> RAKVAMSHFEPHEYIRYDLLEKNIDIVRKRLNRPLTLSEKIVYGHLDDPANQEIERGKTYLRLRPDRVAMQDATAQMAMLQFISSGLPKVAVPSTIHCDHLIEAQLGGEKDLRRAKDINQEVYNFLATAGAKYGVGFWRPGSGIIHQIILENYAYPGVLLIGTDSHTPNGGGLGGICIGVGGADAVDVMAGIPWELKCPKVIGVKLTGSLSGWTSPKDVILKVAGILTVKGGTGAIVEYHGPGVDSISCTGMATICNMGAEIGATTSVFPYNHRMKKYLSKTGRADIANLADEFKDHLVPDPGCHYDQVIEINLSELKPHINGPFTPDLAHPVAEVGSVAEKEGWPLDIRVGLIGSCTNSSYEDMGRSAAVAKQALAHGLKCKSQFTITPGSEQIR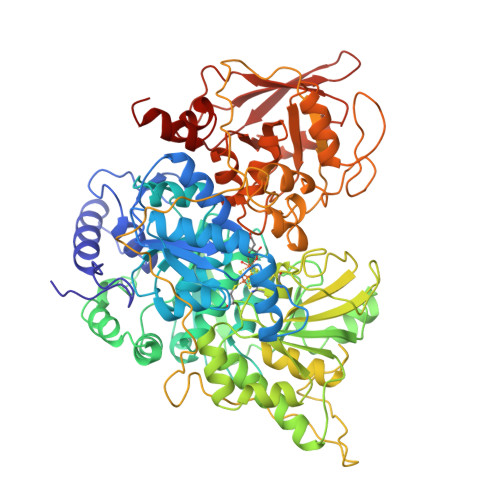ATIERDGYAQVLRDVGGIVLANACGPCIGQWDRKDIKKGEKNTIVTSYNRNFTGRNDANPETHAFVTSPEIVTALAIAGTLKFNPETDFLTGKDGKKFKLEAPDADELPRAEFDPGQDTYQHPPKDSSGQRVDVSPTSQRLQLLEPFDKWDGKDLEDLQILIKVKGKCTTDHISAAGPWLKFRGHLDNISNNLLIGAINIENRKANSVRNAVTQEFGPVPDTARYYKQHGIRWVVIGDENYGEGASREHSALEPRHLGGRAIITKSFARIHETNLKKQGLLPLTFADPADYNKIHPVDKLTIQGLKDFAPGKPLKCIIKHPNGTQETILLNHTFNETQIEWFRAGSALNRMKELQQK>KEDELDSLNEKLKIEHAKKKRLFDLYINGSYEVSELDSMMNDIDAQINY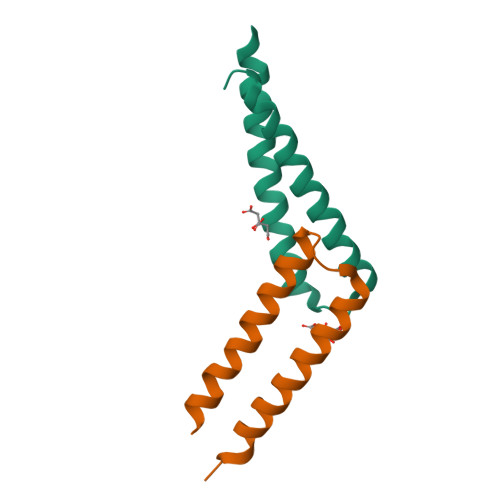YEAQIEANEELKK[4x]>LGVQGLTEEQRMMIRELMDAQMKTFDTTFSHFKNFRLPGVLSSGCELPESLQAPSREEAAKWSQVRKDLCSLKVSLQLRGEDGSVWNYKPPADSGGKEIFSLLPHMADMSTYMFKGIISFAKVISYFRDLPIEDQISLLKGAAFELCQLRFNTVFNAETGTWECGRLSYCLEDTAGGFQQLLLEPMLKFHYMLKKLQLHEEEYVLMQAISLFSPDRPGVLQHRVVDQLQEQFAIT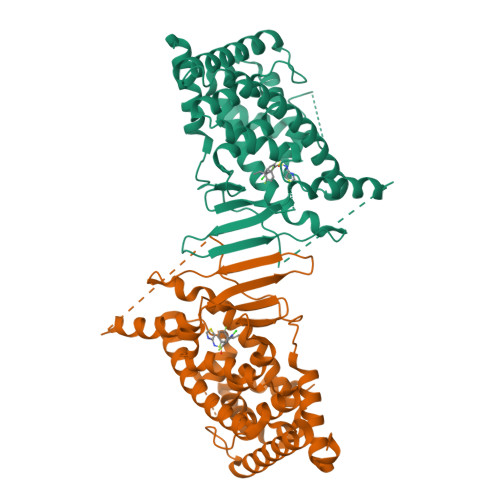LKSYIECNRPQPAHRFLFLKIMAMLTELRSINAQHTQRLLRIQDIHPFATPLMQELFGITGSGGSGGSSHSSLTERHKILHRLLQEGS[2x]Cobra cytotoxins (CTs) belong to the three-fingered protein family and possess membrane activity. Three-finger toxins (TFTs) are disulfide-rich proteins from the venoms of cobras, kraits, coral, and some other snakes. Their fold features three distinct β-structural “fingers”, emerging from a globular core stapled by four conserved disulfide bridges. Cardiotoxins, or cytotoxins (CTs), are one of the largest groups of TFTs, affecting the integrity of lipid membranes, and/or influencing the activity of membrane proteins and the associated signaling cascades. For the first time, a spatial model of CT13Nn with both “water” and “membrane” conformations of the central loop (loop-2) were determined by X-ray crystallography.

Structures of hexagonal (with three molecules in the asymmetric unit denoted A, B, and C) and orthorhombic (with six molecules in an asymmetric unit denoted A, B, C, D, E, and F) crystal forms were solved at 2.3 and 2.6 Å-resolution, respectively. Analysis of the 2Fo-Fc electron density map of the 2.3Å structure revealed that the correct variant is the LLVK sequence. The average value of the B-factor of protein atoms amounts to 38.9 Å2 and 98.5 Å2 in the hexagonal and the orthorhombic form, respectively. This indicates that the hexagonal form is more ordered. The most ordered molecules in the hexagonal and the orthorhombic structure are B and A, respectively. Subunit B of the hexagonal form was further used for conformational analysis and comparison with other NMR or X-ray structures. A root-mean-square deviation (RMSD) between coordinates of Cα atoms of molecule B in the hexagonal crystal form superimposed on the other two molecules ranges from 0.26 to 0.34 Å. Unusual conformation of the loop-2 in all subunits of the hexagonal and most subunits of the orthorhombic form was similar to that found by NMR for cytotoxin 1 from N. oxiana (5NQ4) in DPC micelle. For the first time, in this work the structure similar to the membrane-bound conformation of functionally important loop-2 of an S-type CT was observed in the two crystal forms. Apparently, these conformational changes are caused by the repulsion of loop-2 from its neighbor molecules in the crystal cell.

>LKCNKLIPLAYKTCPAGKNLCYKMFMVSNKTVPVKRGCIDVCPKNSLLVKYVCCNTDRCN[3x]> MKTLVHVASVEKGRSYEDFQKVYNAIALKLREDDEYDNYIGYGPVLVRLAWHTSGTWDKHDNTGGSYGGTYRFKKEFNDPSNAGLQNGFKFLEPIHKEFPWISSGDLFSLGGVTAVQEMQGPKIPWRCGRVDTPEDTTP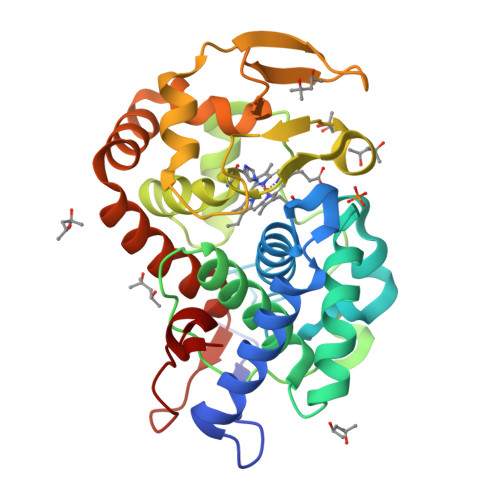DNGRLPDADKDADYVRTFFQRLNMNDREVVALMGAHALGKTHLKNSGYEGPWGAANNVFTNEFYLNLLNENWKLEKNDANNEQWDSKSGYMMLPTDYSLIQDPKYLSIVKEYANDQDKFFKDFSKAFEKLLENGITFPKDAPSPFIFKTLEEQGL> MELKNSISDYTEAEFVQLLKEIEKENVAATDDV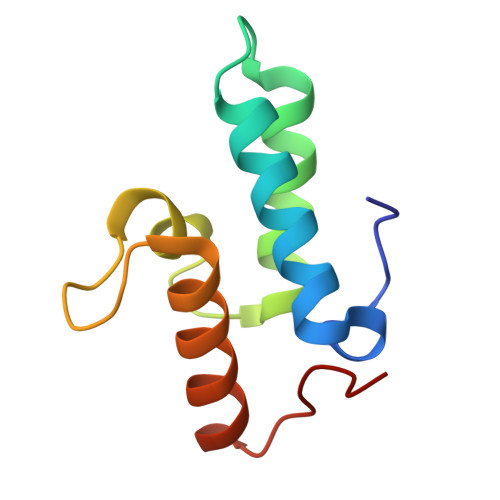LYVLLEHFVKITEHPDGQDLIYYPSDNRDDSPEGIVKEIKEWRAANGKPGFKQG> MQSTLVIAEHANDSLAPITLNTITAATRLGGEVSCLVAGTKCDKVAQDLCKVAGIAKVLVAQHDVYKGLLPEELTPLILATQKQFNYTHICAGASAFGKNLLPRVAAKLEVAPISDIIAIKSPDTFVRTIYAGNALCTVKCDEKVKVFSVRGTSFDAAATSGGSASSEKASSTSPVEISEWLDQKLTKSDRPELTGAKVVVSGGRGLKSGENFKLLYDLADQLHAAVGASRAAVDAGFVPNDMQVGQTGKIVAPELYIAVGISGAIQHLAGMKDSKTIVAINKDPEAPIFQVADYGIVADLFKVVPEMTEILKKK;> MAELRVLVAVKRVIDYAVKIRVKPDRTGVVTDGVKHSMNPFCEIAVEEAVRLKEKKLVKEVIAVSCGPAQCQETIRTALAMGADRGIHVEVPPAEAERLGPLQVA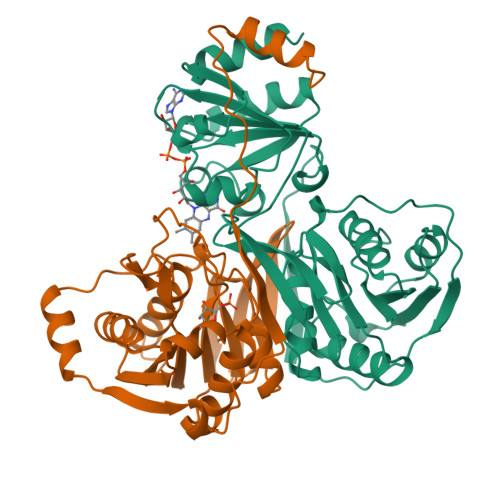RVLAKLAEKEKVDLVLLGKQAIDDDCNQTGQMTAGFLDWPQGTFASQVTLEGDKLKVEREIDGGLETLRLKLPAVVTADLRLNEPRYATLPNIMKAKKKKIEVIKPGDLGVDLTSKLSVISVEDPPQRTAGVKVETTEDLVAKLKEIGRI>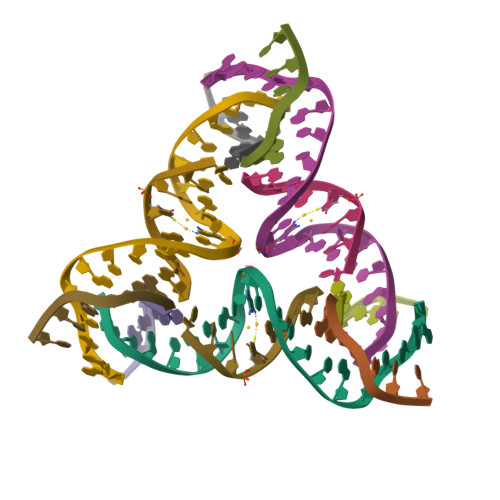 GAGCAGCCTGTATGGACATCA;> CCAXACA;> GGCTGCT;> CTGATGT>[2x]MSMSDINKNSELIFIPAPGIGHLASALEFAKLLTNHDKNLYITVFCIKFPGMPFADSYIKSVLASQPQIQLIDLPEVEPPPQELLKSPEFYILTFLESLIPHVKATIKTILSNKVVGLVLDFFCVSMIDVGNEFGIPSYLFLTSNVGFLSLMLSLKNRQIEEVFDDSDRDH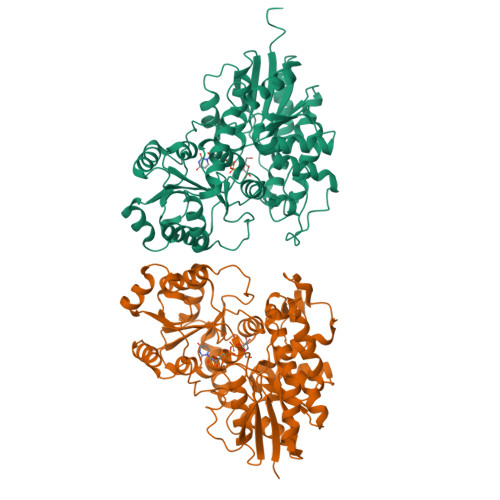QLLNIPGISNQVPSNVLPDACFNKDGGYIAYYKLAERFRDTKGIIVNTFSDLEQSSIDALYDHDEKIPPIYAVGPLLDLKGQPNPKLDQAQHDLILKWLDEQPDKSVVFLCFGSMGVSFGPSQIREIALGLKHSGVRFLWSNSAEKKVFPEGFLEWMELEGKGMICGWAPQVEVLAHKAIGGFVSHCGWNSILESMWFGVPILTWPIYAEQQLNAFRLVKEWGVGLGLRVDYRKGSDVVAAEEIEKGLKDLMDKDSIVHKKVQEMKEMSRNAVVDGGSSLISVGKLIDDITGSN> CAUCCGGUAUCCCAAGACAAUCUUCGGGUUGGGUUGGGAAGUAUCAUGGCUAAUCACCAUGAUGCAAUCGGGUUGAACACUUAAUUGGGUUAAAACGGUGGGGGACGAUCCCGUAACAUCCGUCCUAACGGCGACAGACUGCACGGCCCUGCCUCUUAGGU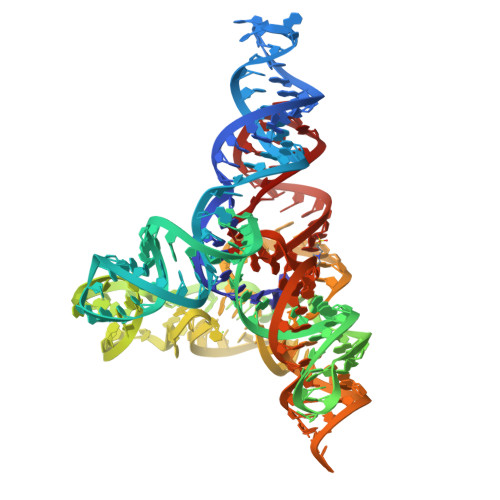GUGUCCAAUGAACAGUCGUUCCGAAAGGAAG> GAGCAGACTTG;> ACAGCACTCA;> CATGT;> TCTGAGTGCAGTCTGC

In this work, we exhaustively probe the ability of all 36 immobile HJ sequences to form DNA crystals in two different designed systems. Three separate self-assembling DNA crystal systems are described in this report: the “4 × 5” and “4 × 6” designs (collectively referred to as the 4 × N systems), and a third construct with a “scrambled” sequence variant of the 4 × 6 lattices. Self-assembly was mediated by three constituent oligonucleotides: (S1) containing four sequence repeats of either 5 or 6 bases; (S2) composed of 21 bases containing complementary regions to both (S1); and (S3) which forms the second junction crossover. The HJ serves as the fundamental component at the core of each unit, and the ultimate assembly of the full lattice is facilitated by the complementary 2-base sticky ends that tail each duplex.

We hypothesized that it might be possible to introduce other unique immobile sequences that could provide slight perturbations in the junction angle, to potentially reduce the strain in the original system and yield a “relaxed,” periodic lattice. The 4 × 5 system robustly crystallized with 75% of the junctions, and we obtained crystals in all but 9 of 36 sequences. Of the resulting structures, 18 exhibited P32 symmetry with average cell dimensions a = b = 68.85 Å c = 60.09 Å, with only nine retaining the original P3221 symmetry with average cell edges a = b = 68.17 Å c = 60.60 Å. Although the cell parameters between the two symmetries were virtually indistinguishable, the differences between the periodicity of the lattices is dramatic, with vastly different cavity sizes. While the highest resolution achieved for the J1 system was 3.1 Å, in roughly half of the crystals measured the resolutions were 3.05 Å or better, and as high as 2.9 Å (J6) and 2.75 Å (J19), for the P32 and P3221 symmetries, respectively. The mean angles across all junctions within the groups were 56.05° (σ = 1.63) and 56.59° (σ = 1.50) for the P32 and P3221, respectively. We hypothesize that even a small difference in junction angles could have a significant global effect on the assembly of the lattice, thereby eliminating the strain in the P3221 lattices.>[2x]GMSSVTWAPGNYPSTRRSDHVDTYQSASKGEVPVPDPYQWLEESTDEVDKWTTAQADLAQSYLDQNADIQKLAEKFRASRNYAKFSAPTLLDDGHWYWFYNRGLQSQSVLYRSKEPALPDFSKGDDNVGDVFFDPNVLAADGSAGMVLCKFSPDGKFFAYAVSHLGGDYSTIYVRSTSSPLSQASVAQGVDGRLSDEVKWFKFSTIIWTKDSKGFLYQRYPARERHEGTRSDRNAMMCYHKVGTTQEEDIIVYQDNEHPEWIYGADTSEDGKYLYLYQFKDTSKKNLLWVAELDEDGVKSGIHWRKVVNEYAADYNIITNHGSLVYIKTNLNAPQYKVITIDLSKDEPEIRDFIPEEKDAKLAQVNCANEEYFVAIYKRNVKDEIYLYSKAGVQLTRLAPDFVGAASIANRQK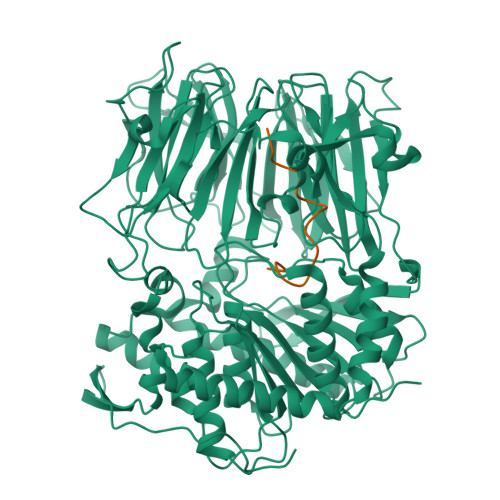QTHFFLTLSGFNTPGTIARYDFTAPETQRFSILRTTKVNELDPDDFESTQVWYESKDGTKIPMFIVRHKSTKFDGTAAAIQYGYGGFATSADPFFSPIILTFLQTYGAIFAVPSIRGGGEFGEEWHKGGRRETKVNTFDDFIAAAQFLVKNKYAAPGKVAINGAANGGLLVMGSIVRAPEGTFGAAVPEGGVADLLKFHKFTGGQAWISEYGNPSIPEEFDYIYPLSPVHNVRTDKVMPATLITVNIGDGRVVPMHSFKFIATLQHNVPQNPHPLLIKIDKSWLGHGMGKPTDKNVKDAADKWGFIARALGLELKTVE;>IWGIGCNPWTAEHVDQTLASGNDIC[2x]>[2x]MSIVVKNNIHWVGQRDWEVRDFHGTEYKTLRGSSYNSYLIREEKNVLIDTVDHKFSREFVQNLRNEIDLADIDYIVINHAEEDHAGA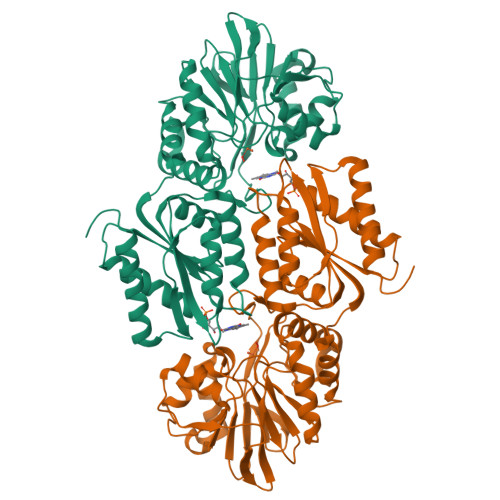LTELMAQIPDTPIYCTANAIDSINGHHHHPEWNFNVVKTGDTLDIGNGKQLIFVETPMLHWPDSMMTYLTGDAVLFSNDAFGQHYCDEHLFNDEVDQTELFEQCQRYYANILTPFSRLVTPKITEILGFNLPVDMIATSHGVVWRDNPTQIVELYLKWAADYQEDRITIFYDTMYNNTRMMADAIAQGIAETDPRVAVKIFNVARSDKNEILTNVFRSKGVLVGTSTMNNVMMPKIAGLVEEMTGLRFRNKRASAFGSHGWSGGAVDRLSTRLQDAGFEMSLSLKAKWRPDQDALKLCREHGREIARQWALAPLPQSTVNTVVKEETSATTTADLGPRMQCSVCQWIYDPAKGEPMQDVAPGTPWSEVPDNFLCPECSLGKDVFEELASEAK> QAEEWYFGKITRRESERLLLNPEN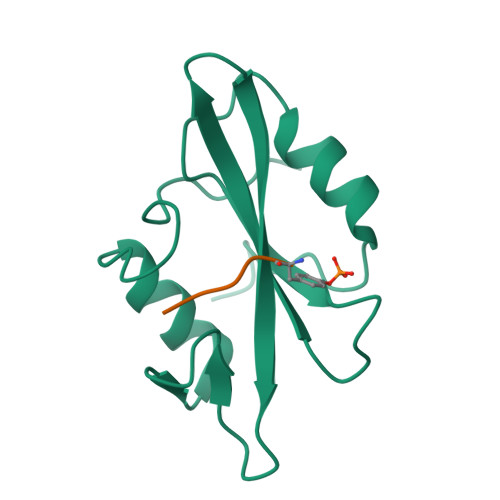PRGTFLVRESETTKGAYCLSVSDFDNAKGLNVKHYKIRKLDSGGFYITSRTQFSSLQQLVAYYSKHADGLCHRLTNVCPT;> YLRVA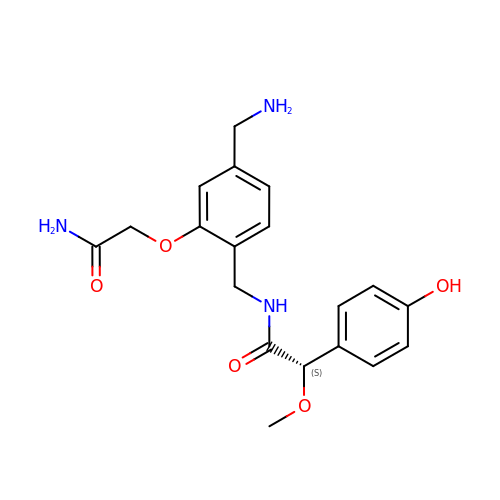(2~{S})-~{N}-[[4-(aminomethyl)-2-(2-azanyl-2-oxidanylidene-ethoxy)phenyl]methyl]-2-(4-hydroxyphenyl)-2-methoxy-ethanamide | C19 H23 N3 O5 | ZCVNZLWWFYCDGA-SFHVURJKSA-N> MGSSHHHHHHSSGRENLYFQGPSNSDAAHAFWSTQPVPQTEDEDEKIVFAGPMDEPKTV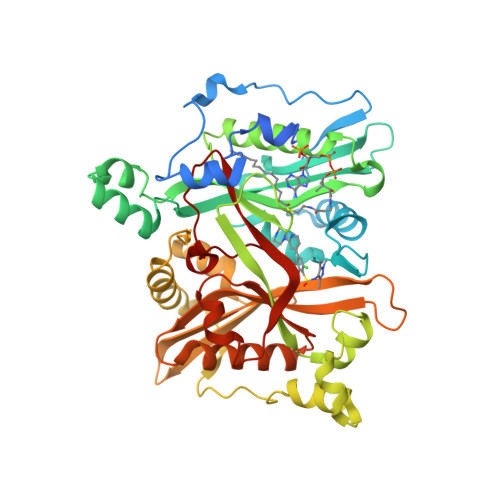ADIPEEPYPIASTFEWWTPNMEAADDIHAIYELLRDNYVEDDDSMFRFNYSEEFLQWALCPPNYIPDWHVAVRRKADKKLLAFIAGVPVTLRMGTPKYMKVKAQEKGEGEEAAKYDEPRHICEINFLCVHKQLREKRLAPILIKEATRRVNRTNVWQAVYTAGVLLPTPYASGQYFHRSLNPEKLVEIRFSGIPAQYQKFQNPMAMLKRNYQLPSAPKNSGLREMKPSDVPQVRRILMNYLDSFDVGPVFSDAEISHYLLPRDGVVFTYVVENDKKVTDFFSFYRIPSTVIGNSNYNLLNAAYVHYYAATSIPLHQLILDLLIVAHSRGFDVCNMVEILDNRSFVEQLKFGAGDGHLRYYFYNWAYPKIKPSQVALVML[(1S)-1-{[(2-benzylphenyl)carbonyl]amino}ethyl](trihydroxy)borate(1-) | C16 H19 B N O4 | 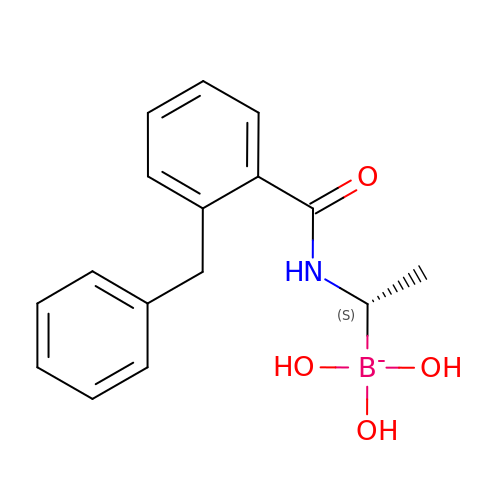KXUAFLYMMJHXHZ-GFCCVEGCSA-N>TYTISIRVYQTTPKGFFRPVERTNWKYANGGTWDEVRGEYVLTMGGSGTSGSLRFVSSDTDESFVATFGVHNYKRWCDIVTNLTNEQTALVINQEYYGVPIRDQARENQLTSY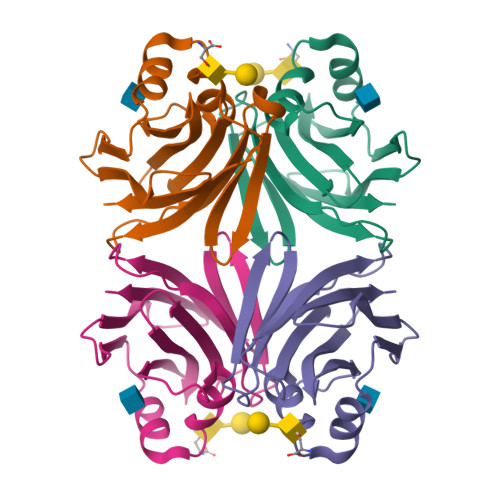NVANAKGRRFAIEYTVTEGDNLKANLIIG[4x]2-({[4-(methylsulfanyl)phenyl]methyl}amino)ethan-1-ol 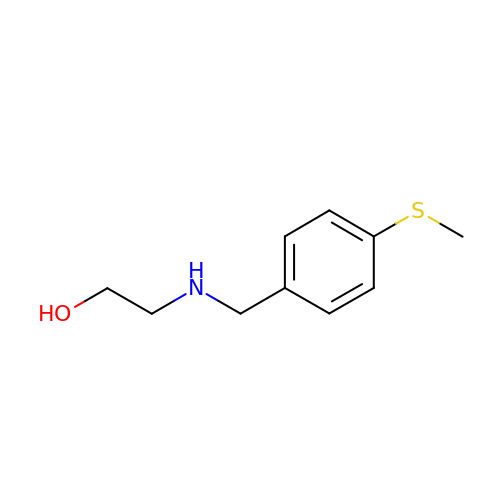| C10 H15 N O S | MXNHNDNJEDGUBO-UHFFFAOYSA-N> MAPVKVFGPAMSTNVARVTLCLEEVGAEYEVVNIDFNTMEHKSPEHLARNPFGQIPAFQDGDLLLWESRAISKYVLRKYKTDEVDLLRESNLEEAAMVDVWTEVDAHTYNPALSPIVYQCLTNPMMRGLPTDEKVVAESLEKLKKVLEVYEARLSKHSYLAGDFV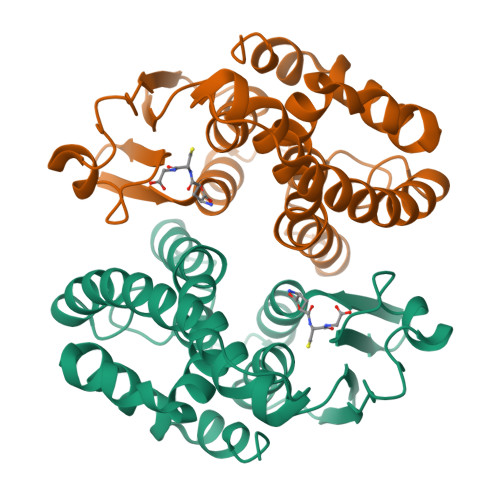SFADLNHFPYTFYFMATPHAALFDSYPHVKAWWDRLMARPAVKKIAATMVPPKA>GIGKFLHAAKKFXKAFVAEIMNS[2x];>[2x]GIGKFLHAAKKFAKAFVAEIMN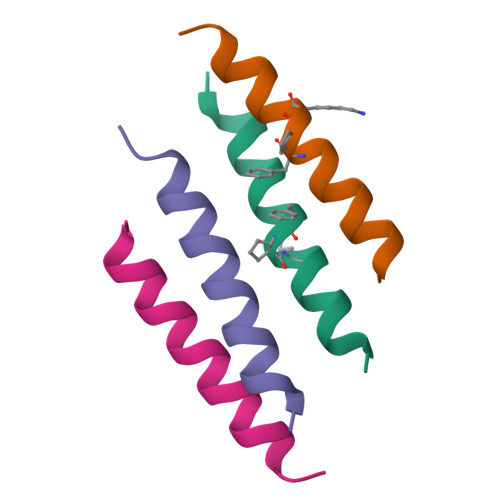S>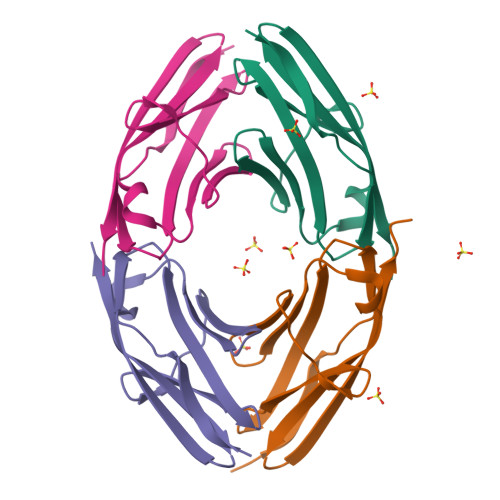[4x]HPPPTDSTLRPMFKRLLANAECQEGQSVCFEIRVSGIPPPTLKWEKDGQPLSLGPNIEIIHEGLDYYALHIRDTLPEDTGYYRVTATNTAGSTSCQAHLQVERLR> MREYKLVVLGSGGVGKSALTVQFVQGIFVEKYDPTIEDSYRKQVEVDAQQCMLEILDTAGTEQFTAMRDLYMKNGQGFALVYSITAQSTFNDLQDLREQILRVKDTDDVPMILVGNKCDLEDERVVGKEQGQNLARQWNNC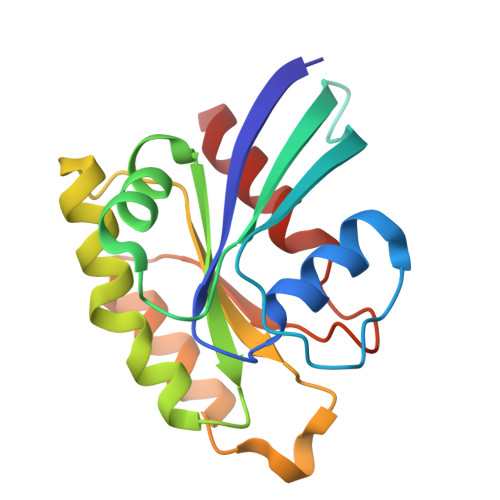AFLESSAKSKINVNEIFYDLVRQINR4-bromanyl-2-methyl-pyrazol-3-amine 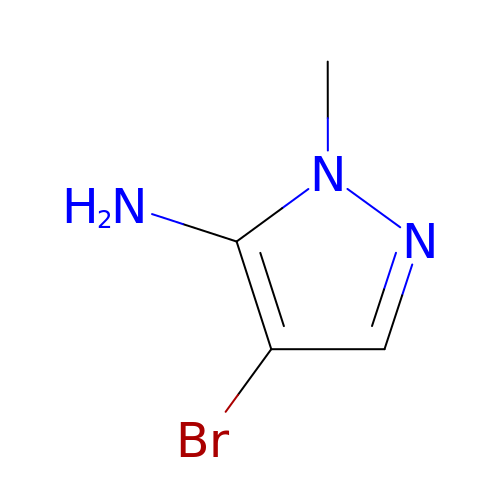| C4 H6 Br N3 | ODFDZOQJRPDQDF-UHFFFAOYSA-N2-[4-[4-[[(6Z)-5-chloranyl-6-pyrazolo[1,5-a]pyridin-3-ylidene-1H-pyrimidin-2-yl]amino]-3,5-dimethyl-pyrazol-1-yl]piperidin-1-yl]-N,N-dimethyl-ethanamide 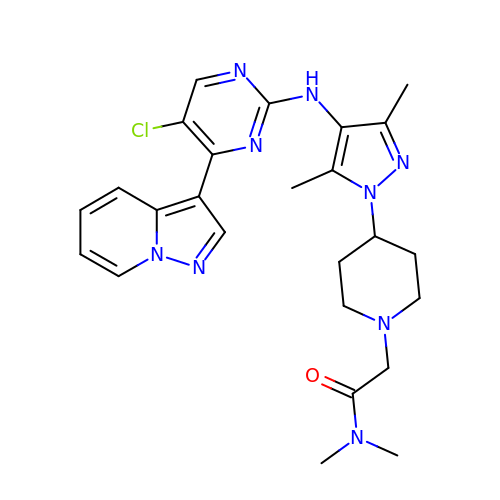| C25 H30 Cl N9 O | FDWQWRCUIAECJN-UHFFFAOYSA-N> DKSGMKSIDT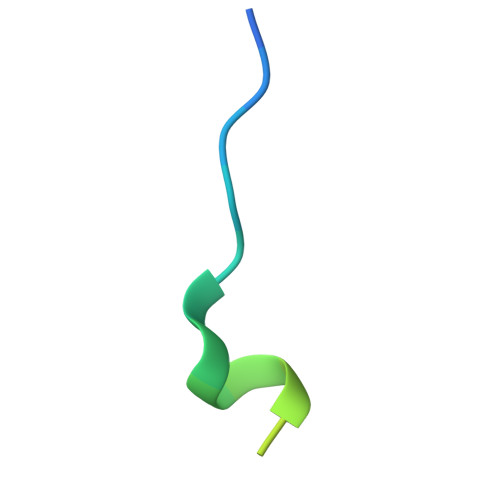FFGVKNKKKIGKV>[2x]MRGSHHHHHHGSIKKPINVAIFGSTGSIGTNALNIIRECNKIENVFNVKALYVNKSVNELYEQAREFLPEYLCIHDKSVYEELKELVKNIKDYKPIILCGDEGMKEICSSNSIDKIVIGIDSFQGLYSTMYAIMNNKIVALANKESIVSAGFFLKKLLNIHKNAKIIPVDSEHSAIFQCLDN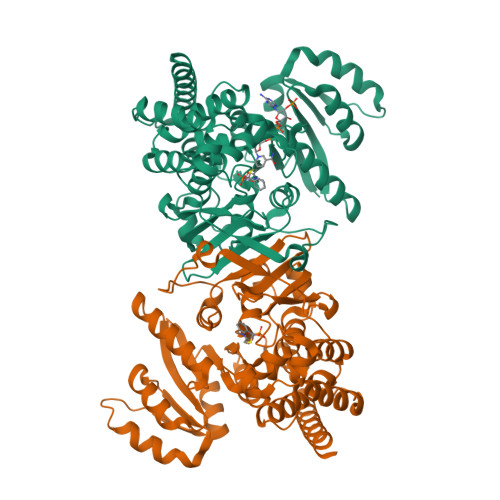NKVLKTKCLQDNFSKINNINKIFLCSSGGPFQNLTMDELKNVTSENALKHPKWKMGKKITIDSATMMNKGLEVIETHFLFDVDYNDIEVIVHKECIIHSCVEFIDKSVISQMYYPDMQIPILYSLTWPDRIKTNLKPLDLAQVSTLTFHKPSLEHFPCIKLAYQAGIKGNFYPTVLNASNEIANNLFLNNKIKYFDISSIISQVLESFNSQKVSENSEDLMKQILQIHSWAKDKATDIYNKHNSS~{N}-[(1~{S})-1-(4-fluorophenyl)-1-[2-[4-[6-(1-methylpyrazol-4-yl)pyrrolo[2,1-f][1,2,4]triazin-4-yl]piperazin-1-yl]pyrimidin-5-yl]ethyl]ethanamide 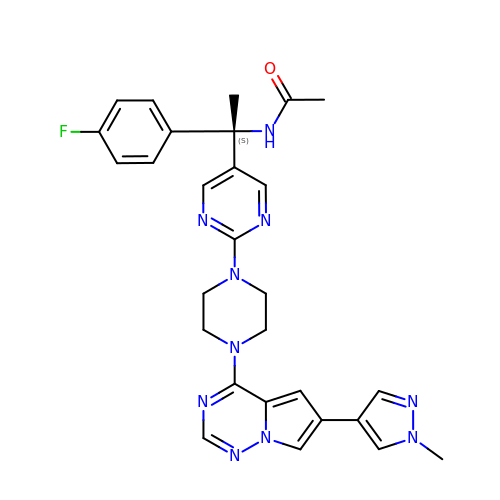| C28 H29 F N10 O | JWBYZGLZBJQWBU-NDEPHWFRSA-N>[4x]QSSNLSSDAVIGSIAQGVTDGLTDYLKPRVEELPAGEVTYPEIAGLPDGVRVISAEWATSKHVILTIQSAAMPERPIKVQLLLPRDWYSSPNREFPEIWALDGLRAIEEQSGWTIETNIEQYYADKNAIVVLPVGGESSFYSDWEGPNNGKNYQWETFLTQELAPILDKGFRSNTDRAITGISMGGTAAVNIATHHPDMFKFVGSFSGYLDTTSAGMPIAISAALADAGGYDANAMWGPVGSERWQENDPKSNVDKLKGKTIYVSSGNGADDFGKEGSVAIGPANAAGVGLE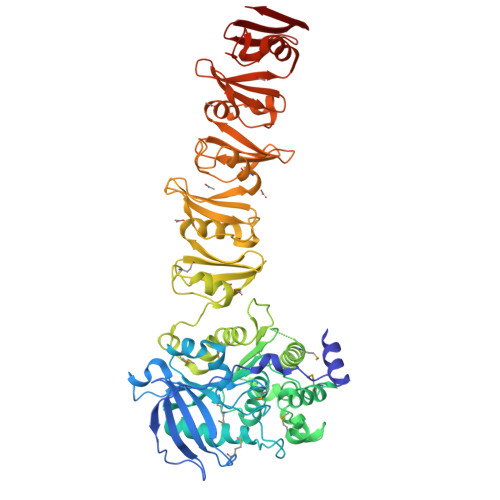VISRMTSQTFVDRASQAGVEVVASFRPSGVHSWEYWQFEMTQAFPHIANALGMSTEDRGVECAPVGAIADAVADGAMGTCLTNEYDVTGGKAQDFANGRAYWSANTGAFGLVGRINARYSELGGPASWLGYPTSSELKTPDGRGRFVTFEHGSIYWTATTGPWEIPGDMLAAWGTQDYEKGSLGYPTGAAVEYNGGLRQQFEGGYVFRTSNNQSYWVRGEISKKYAEDGIFAQLGFPTGNEKLINGGAFQEFEKGNIYWSASTGAHVILHGDIFDAWGAKGWEQGEYGFPTSDQTAITAGGQTIDFQNGTIRQVNGRIEESRHHHHHH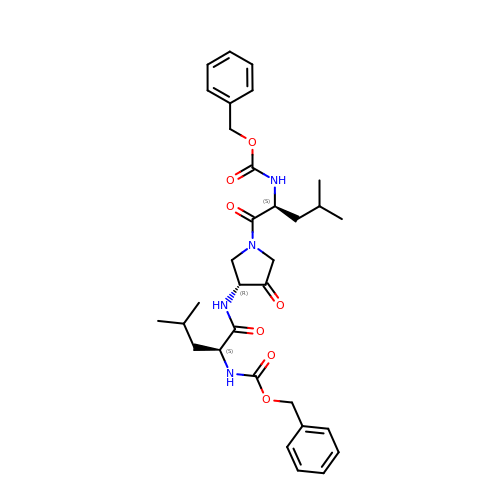1-[N[(PHENYLMETHOXY)CARBONYL]-L-LEUCYL-4-[[N/N-[(PHENYLMETHOXY)CARBONYL]-/NL-LEUCYL]AMINO]-3-PYRROLIDINONE/N | C32 H42 N4 O7 | GXENQLUSOCKXDN-GMQQYTKMSA-N>SMLSAASRVVSRAAVHCALRSPPPEARALAMSRPPPPRVASVLGTMEMGRRMDAPASAAAVRAFLERGHTELDTAFMYSDGQSETILGGLGLGLGGGDCRVKIATKANPWDGKSLKPDSVRSQLETSLKRLQCPQVDLFYLHAPDHGTPVEETLHACQRLHQEGKFVELGLSNYASWEVAEICTLCKSNGWILPTVYQGMYNATTRQVETELFPCLRHFGLRFYAYNPLAGGLLTGKYKYEDKDGKQPVGRFFGNSWAETYRNRFWKEHHFEA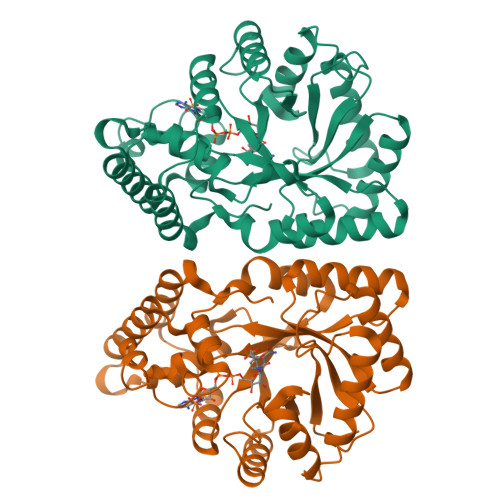IALVEKALQAAYGASAPSVTSAALRWMYHHSQLQGAHGDAVILGMSSLEQLEQNLAATEEGPLEPAVVDAFNQAWHLVAHECPNYFR[4x]1,4-BUTANEDIOL | C4 H10 O2 | 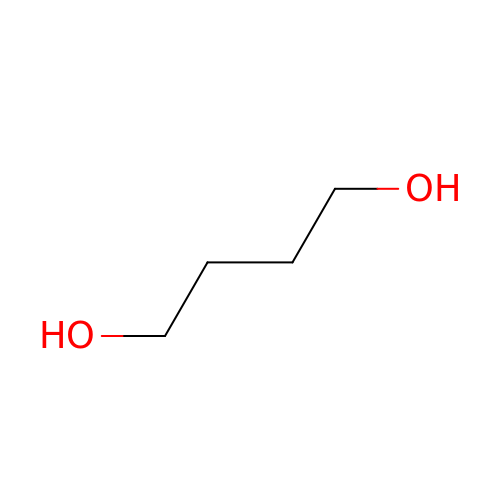WERYXYBDKMZEQL-UHFFFAOYSA-N>[4x]GMTDRLKGKVAIVTGGTLGIGLAIADKFVEEGAKVVITGRHADVGEKAAKSIGGTDVIRFVQHDASDEAGWTKLFDTTEEAFGPVTTVVNNAGIAVSKSVEDTTTEEWRKLLSVNLDGVFFGTRLGIQRMKNKGLGASIINMSS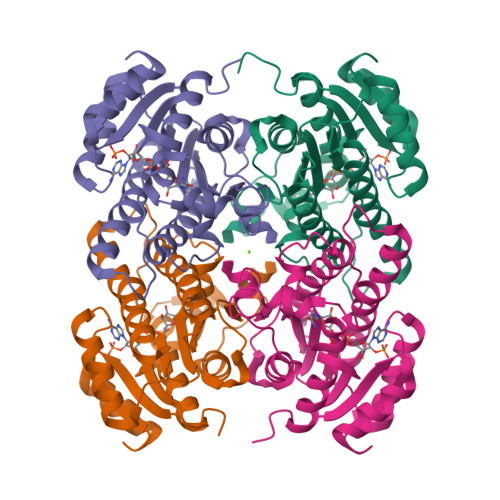IEGLVGDPTQGAYNASKGAVRIMSKSAALDCALKDYDVRVNTVHPGPIKTPLVDDAEGAEEFFSQRTKTPMGHIGEPNDIAWICVYLASDESKFATGAEFVVDGGYTAQ2-{5-[(4-chloro-2-methylphenyl)methoxy]-1H-pyrazol-1-yl}pyridine-4-carboxylic 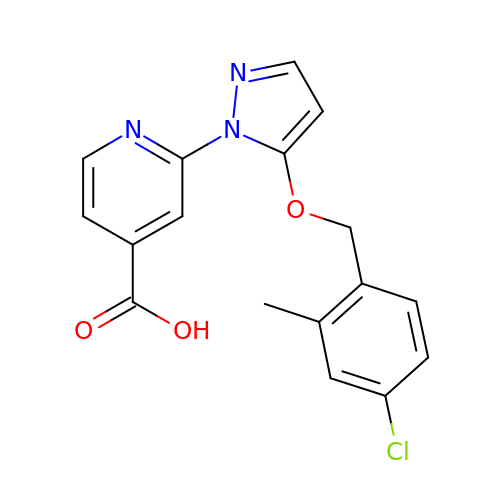acid | C17 H14 Cl N3 O3 | PSOBPHXKKHPWMU-UHFFFAOYSA-N3-{[(14beta,16alpha,17alpha)-3-(2-bromoethyl)-17-hydroxyestra-1,3,5(10)-trien-16-yl]methyl}benzamide 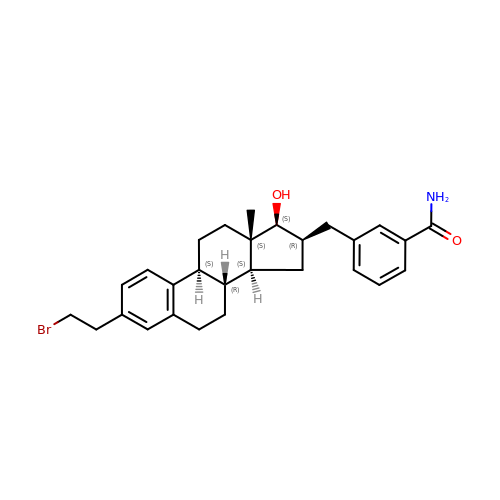| C28 H34 Br N O2 | LSFSILMVQQMGRP-OPRSCSRJSA-N> LYI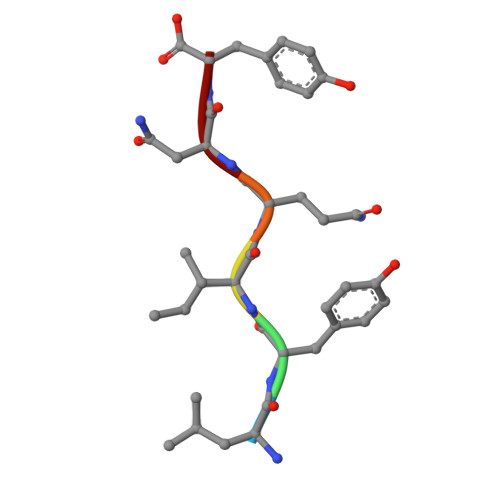QNY Copper transporting P-type ATPase proteins are key regulators of cellular copper and are found in all kingdoms of life. To further dissect the transport and regulation mechanisms of P1B-1-ATPases, we focused on a member from rice (Oryza sativa), OsHMA4, or simply HMA49. This protein is localized to the tonoplasts of roots, and is involved in root-to-shoot translocation and grain accumulation of copper. HMA4 has three predicted N-terminal ferredoxin-like MBDs, although the one closest in sequence to the M-domain and the P-type ATPase core, MBD−1, lacks the metal-binding CXXC-motif.

The protein was produced and purified from Saccharomyces cerevisiae, frozen on grids in the presence of detergent and with one of the established state stabilizing phosphate mimics BeF3- or AlF4- that inhibit protein function. These have previously been used to trap the outward-open E2P conformation, and an outward-facing (E2.Pi) transition state of dephosphorylation, respectively. We also studied the effect of no such supplementation to HMA4, which has previously yielded an early E1 state of AfCopA26. These various conditions yielded four structures, determined at overall resolutions of 3.3 (HMA4BeF), 3.2 (HMA4AlF), 3.6 (HMA4apo), and 3.7 Å (HMA4Cu). Inspection of the cryo-EM HMA4BeF and HMA4AlF maps and models suggest BeF3− or AlF4− associated with the TGE- and DKTGT-motifs, starting with T480 and D641, respectively. However, in HMA4BeF/HMA4AlF the M3 transmembrane segment is partly covering the MB’ platform, and the two cysteines of the invariant CPC-motif of M4 are further away from the intracellular surface than in HMA4apo/HMA4Cu, indicative of an architecture less compatible with receiving metal. On the other side of the membrane, an outside-exposed pathway is present in HMA4BeF and HMA4AlF, but not in the other two structures. Equivalently, the position of the omnipresent TGE- and DKTGT-motifs in the soluble domains shift from distant in HMA4apo/HMA4Cu to adjacent to each other in HMA4BeF/HMA4AlF, the latter representing a requirement to permit dephosphorylation. Collectively, these observations suggest the HMA4BeF/HMA4AlF structures represent early E2 conformations linked to copper release, likely E2P, while the HMA4apo/HMA4Cu rather represent early E1 states associated with copper uptake. In HMA4BeF/HMA4AlF an outward-open, water-accessible conduit reaches the CPC motif cysteines. From there and to the extracellular side, the pathway is lined by residues of MA, M2 and M6: including M941, M391, M292, E387, M295, D384 and M319, of which M295, E387, M391, and M941 are highly conserved.

> EVDELQEQEIAVCRLQIKGMACTSCSESVERALQMVPGVKKAAVGLALEEAKVHFDPNITSRDLIIEAIEDAGFGADLISSGDDVNKVHLKLEGVSSPEDIKLIQSRLESVEGVNNVECDTAGQTIIVAYDPDVTGPRLLIQCIQDAAQPPKYFNASLYSPPKQREAERHHEIRNYRNQFLWSCLFSVPVFMFSMVLPMISPFGDWLFYKVCNNMTIGMLLRWLLCSPVQFIIGWRFYVGAYHALKRGYSNMDVLVALGTNAAYFYSVYIVLKALTSESFEGQDFFETSAMLISFILLGKYLEVVAKGKTSDALSKLTELAPETACLLTLDKDGNAISETEISTQLLQRNDVIKIVPGEKVPVDGVVIKGQSHVNESMITGEARPIAKKPGDKVIGGTVNDNGCIIVKVTHVGSETALSQIVQLVEAAQLARAPVQKLADRISRFFVPTVVVAAFLTWLGWFVAGQFDIYPREWIPKAMDSFELALQFGISVLVVACPCALGLATPTAVMVATGKGASQGVLIKGGNALEKAHKVKAIIFDKTGTLTVGKPSVVQTKVFSKIPLLELCDLAAGAEANSEHPLSKAIVEYTKKLREQYGSHSDHIMESKDFEVHPGAGVSANVEGKLVLVGNKRLMQEFEVPISSEVEGHMSETEELARTCVLVAIDRTICGALSVSDPLKPEAGRAISYLSSMGISSIMVTGDNWATAKSIAKEVGIGTVFAEIDPVGKAEKIKDLQMKGLTVAMVGDGINDSPALAAADVGLAIGAGTDVAIEAADIVLMRSSLEDVITAIDLSRKTLSRIRLNYVWALGYNVLGMPVAAGVLFPFTGIRLPPWLAGACMAASSVSVVCSSLLLQLYKKPLHVEEVAAGPKNDPDLV>GHMSEVLPAGLATTVLVPASSANLGPGFDSLGIALSLYDEIEV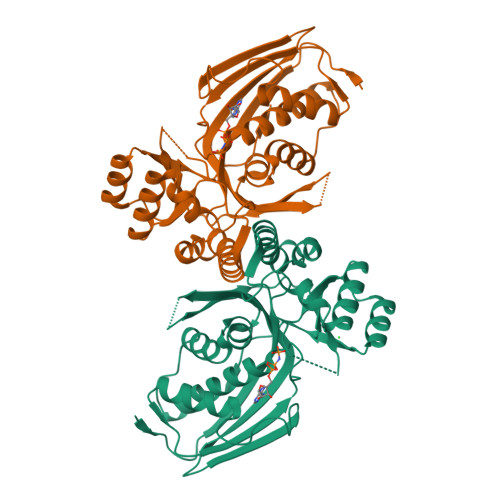NTTESGLKVAVEGQGAGEVPLDGSHLVVRAIERGLAAGGAAAPGLIVQCHNKIPHSRGLGSSAAAAVAGLGVANGLLAKAGRAVLSDDVLVQLASEFEGHPDNAAASVLGGAVVSWSETSGATPIYAATRLDVHPDIKIVAAIPEEQSSTAHTRVLLPQAVTHVDARFNISRVALLTVALTARPDLLMTATEDRLHQPQRASAMPASADVLAYLRSQGVAAVLSGAGPAVLALTTVDLPDSAVKYAEDQGFSLVAMAVSAGVSVR[2x]>[2x]SNAMNRTKKAIFEAAINVFATSGYNGSTVDEIASKANVAKGTLYYNFKSKEEIFNFVISKGLEIWHEKLTDIENLEDEPIEKLKKLFKMQFELLYE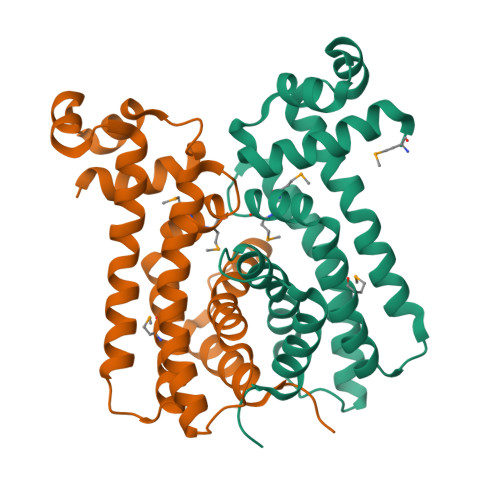NRAFFKMVMSQLWGKETRQDELRNKITEYIEGIERILKEAISKKQIRECDISLLAHSLFGSLISTSLYELSRDKEFNVNKVIDEITINILDGIVIK> DDDD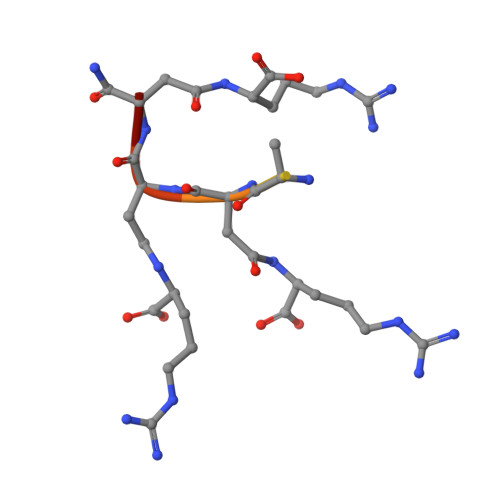DDDDN N-{5-[difluoro(phosphono)methyl]-1-benzothiophene-2-carbonyl}-3-methyl-L-valyl-L-prolyl-N~3~-(1,3-benzothiazol-5-yl)-N,N-dimethyl-beta-alaninamide 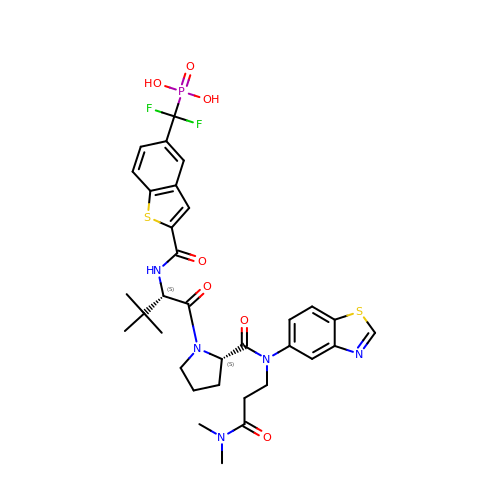| C33 H38 F2 N5 O7 P S2 | GKPJRLZYUBSWJX-NEKDWFFYSA-N>SNAMTDTEQTRALA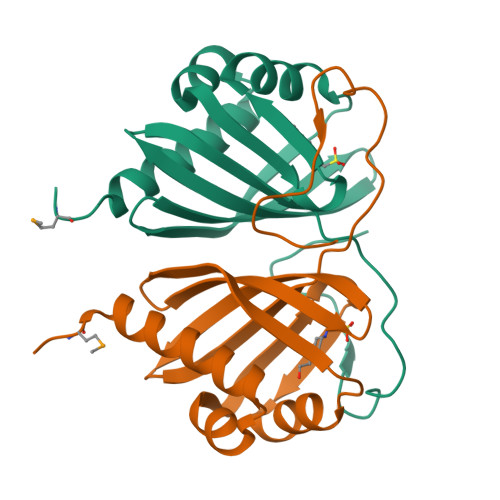RKYFDTLNGRAWEEFAALLAEDVRYELPQTSERITGRADYLRFNQEYPGDWQLTVTRLLADGPSAAVSVNLTLGDERLVGVVFLEVVDGLVSRVTDFWPEAYEPPPGREHLVERVPAELDRFGDS[2x]> MAPKKQEQEPIRLSTRTASKKVDYLQLSNGKLEDFFDDLEEDNKPARNRSRSKKRGRKPLKKADSRSKTPSRVSNARGRSKSLGPRKTYPRKKNLSPDNQLSLLLKWRNDKIPLKSASETDNKCKVVNVKNIFKSDLSKYGANLQALFINALWKVKSRKEKEGLNINDLSNLKIPLSLMKNGILFIWSEKEILGQIVEIMEQKGFTYIENFSIMFLGLNKCLQSINHKDEDSQNSTASTNNTNNEAITSDLTLKDTSKFSDQIQDNHSEDSDQARKQQTPDDITQKKNKLLKKSSVPSIQKLFEEDPVQTPSVNKPIEKSIEQVTQEKKFVMNNLDILKSTDINNLFLRNNYPYFKKTRHTLLMFRRIGDKNQKLELRHQRTSDVVFEVTDEQDPSKVDTMMKEYVYQMIETLLPKAQFIPGVDKHLKMMELFASTDNYRPGWISVIEK;> MSKAVNKKGLRPRKSDSILDHIKNKLDQEFLEDNENGEQSDEDYDQKSLNKAKKPYKKRQTQNGSELVISQQKTKAKASANNKKSAKNSQKLDEEEKIVEEEDLSPQKNGAVSEDDQQQEASTQEDDYLDRLPKSKKGLQGLLQDIEKRILHYKQLFFKEQNEIANGKRSMVPDNSIPICSDVTKLNFQALIDAQMRHAGKMFDVIMMDPPWQLSSSQPSRGVAIAYDSLSDEKIQNMPIQSLQQDGFIFVWAINAKYRVTIKMIENWGYKLVDEITWVKKTVNGKIAKGHGFYLQHAKESCLIGVKGDVDNGRFKKNIASDVIFSERRGQSQKPEEIYQYINQLCPNGNYLEIFARRNNLHDNWVSIGNEL;> MSLKKGKFQHNQSKSLWNYTLSPGWREEEVKILKSALQLFGIGKWKKIMESGCLPGKSIGQIYMQTQRLLGQQSLGDFMGLQIDLEAVFNQNMKKQDVLRKNNCIINTGDNPTKEERKRRIEQNRKIYGLSAKQIAEIKLPKVKKHAPQYMTLEDIENEKFTNLEILTHLYNLKAEIVRRLAEQGETIAQPSIIKSLNNLNHNLEQNQNSNSSTETKVTLEQSGKKKYKVLAIEETELQNGPIATNSQKKSINGKRKNNRKINSDSEGNEEDISLEDIDSQESEINSEEIVEDDEEDEQIEEPSKIKKRKKNPEQESEEDDIEEDQEEDELVVNEEEIFEDDDDDEDNQDSSEDDDDDED;> MKHHHHHHHGAAGTSLYKKAGENLYFQGSMKKNGKSQNQPLDFTQYAKNMRKDLSNQDICLEDGALNHSYFLTKKGQYWTPLNQKALQRGIELF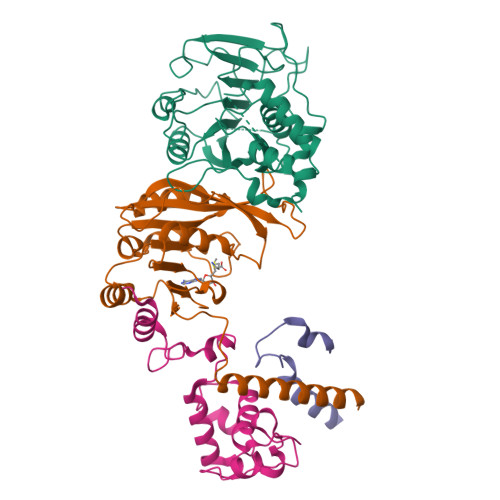GVGNWKEINYDEFSGKANIVELELRTCMILGINDITEYYGKKISEEEQEEIKKSNIAKGKKENKLKDNIYQKLQQMQ> MVTFHTNHGDIVIKTFDDKAPETVKNFLDYCREGFYNNTIFHRVINGFMIQGGGFEPGMKQKATKEPIKNEANNGLKNTRG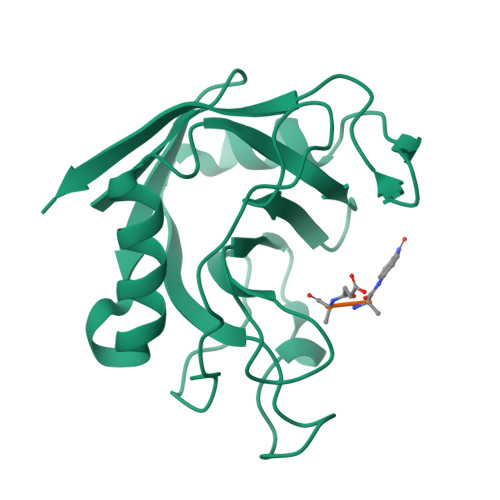TLAMARTQAPHSATAQFFINVVDNDFLNFSGESLQGWGYCVFAEVVDGMDEVDKIKGVATGRSGMHQDVPKEDVIIESVTVSE> ASMTGGQQMGRGSSLTACPEESPLLVGPMLIEFNIPVDLKLVEQQNPKVKLGGRYTPMDCISPHKVAIIIPFRNRQEHLKYWLYYLHPILQRQQLDYGIYVINQAGESMFNKAKLLNVGFKEALKDYDYNCFVFSDVDLIPMNDHNTYRCFSQPRHISVAMDKFGFSLPYVQYFGGVSALSKQQFLSI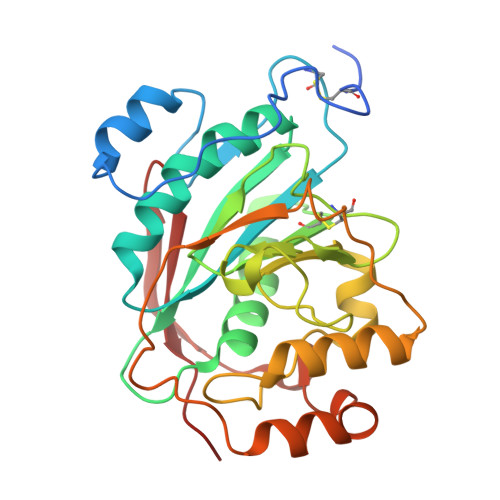NGFPNNYWGWGGEDDDIYNRLAFRGMSVSRPNAVIGKTRMIRHSRDKKNEPNPQRFDRIAHTKETMLSDGLNSLTYMVLEVQRYPLYTKITVDIGTPS Quinol-dependent nitric oxide reductases (qNORs) are membrane-integrated, iron-containing enzymes of the denitrification pathway, which catalyze the reduction of nitric oxide (NO) to the major ozone destroying gas nitrous oxide (N2O). NORs catalyze the reduction of two molecules of nitric oxide (NO) to nitrous oxide (N2O), using two protons and two electrons to cleave the N─O bond and concurrent N─N bond formation: 2NO + 2H+ + 2e− → N2O + H2O. In contrast, qNORs are single subunit enzymes (NorZ), in which electrons are supplied by menaquinol. qNORs are found not only in denitrifying organisms but also in various pathogenic species, many of which lack the full denitrifying apparatus, bringing to attention the role of qNORs in detoxification. Cryo-EM structures unexpectedly revealed AxqNOR to be a dimer.

AxqNOR fused with apocytochrome b562 [BRIL (30)], AxqNOR-BRIL, yielded membrane fractions with high NO consumption rates relative to the total protein content and was chosen for structural studies. Data were processed, with C2 symmetry imposed, providing a structure with a global resolution of 3.9 Å [estimated using the gold standard Fourier shell correlation (FSC) = 0.143 criterion (32)], where local resolution valued the core of the protein calculated at 3.7 Å. Because the BRIL density was at significantly lower resolution, it was omitted during model building, leaving just the AxqNOR model. The dimeric AxqNOR is related by a twofold symmetry axis and exhibits a similar overall structure to those of other qNORs, with 14 transmembrane helices (TMHs) and an α-helical hydrophilic region. The map showed helix pitches and density for bulky side chains, consistent with the estimated resolution, with several hydrophobic interactions between TMHII of each respective molecule, where Leu240, Leu241, and Ile244 act to stabilize the interhelical interaction. The densities of heme b3, FeB, and their respective ligands (His486, His537, His538, and His629) are well defined, where additional conserved residues (Tyr638 and Gly603) provide structural support to Glu490 and His629, respectively. Previous structures of active NORs, including cNOR, have shown the heme b3 Fe to FeB distance to be between 3.2 and 3.9 Å [for NmqNOR and Pseudomonas aeruginosa cNOR (PacNOR), respectively], whereas in AxqNOR, the distance is 4.1 Å. The AxqNOR structure contains the correct nonheme metal at the binuclear center (FeB), but the density for the carboxyl group of Glu490 suggests a different conformation for the side chain compared to GsqNOR and PacNOR, with the carboxyl group approximately 3.5 Å from the His486 NE2 atom. Glu490 in AxqNOR unequivocally faces away from FeB, suggesting that Glu490 and its equivalents in (active) qNORs do not act as an FeB ligand and instead ligate a water molecule along with Glu559. A notable difference was the poor density of Glu494 side chain, which, in the wild-type AxqNOR, was resolved to be facing toward Asn600, forming a hydrogen bond.

>MGPYRRLWFTLIAVLAVTFALLGFYGGEVYRQAPPIPEEVASADGTRLFGRDDILDGQTAWQSIGGMQLGSIWGHGAYQAPDWTADWLHRELMAWLDLAARDAHGRDYGQLDAPAQAALREQLKAEYRANRADAAGGKLTLSPRRAQAVAQTEAYYDQLFSDAPALHRSRENYAMKENTLPDANRRRQMTHFFFWTAWAAGTEREGTSVTYTNNWPHEPLIGNHPSSENVMWSIISVVVLLAGIGLLIWAWAFLRGKEEDEPPAPARDPLTTFALTPSQRALGKYLFLVVALFGFQVLLGGFTAHYTVEGQKFYGIDLSQWFPYSLVRTWHIQSALFWIATGFLAAGLFLAPLINGGRDPKYQKAGVDILFWALVLVVVGSFAGNYLAIAQIMPPDLNFWLGHQGYEYVDLGRLWQIGKFAGICFWLVLMLRGIVPALRTPGGDKNLLALLTASVGAIGLFYGAGFFYGERTHLTVMEYWRWWIVHLWVEGFFEVFATTALAFIFSTLGLVSRRMATTASLASASLFMLGGIPGTFHHLYFAGTTTPVMAVGASFSALEVVPLIVLGHEAWENWRLKTRAPWMENLKWPLMCFVAVAFWNMLGAGVFGFMINPPVSLYYIQGLNTTPVHAHAALFGVYGFLALGFTLLVLRYIRPQYALSPGLMKLAFWGLNLGLALMIFTSLLPIGLIQFHASVSEGMWYARSEAFMQQDILKTLRWGRTFGDVVFLLGALAMVVQVILGLLSGK[2x]>MKNVLVFLILLVALPALAQGHKPLEVIKIEDGVYLHTSFKNIEGYGLVDSNGLVVLDNNQAYIIDTPWSEEDTKLLLSWATDRGYQVMASISTHSHEDRTAGIKLLNSKSIPTYTSELTKKLLAREGKPVPTHYFKDDEFTLGNGLIELYYPGAGHTEDNIVAWLPKSKI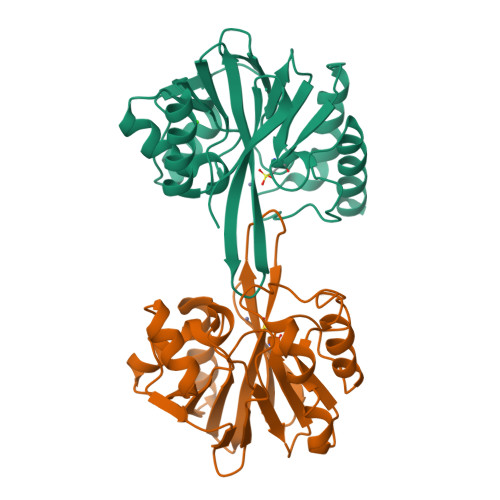LFGGCLVRSHEYEGLGYVGDASISSWADSIKNIVSKKYPIQMVVPGHGKVGSSDILDHTIDLAESASNKLMQPTAEASAD[2x]> MAHHHHHHSLTAYQASSQARVDAAMHTLFTAPSPELARLYEAMRYSVMNGGKRVRPLLAYAACEALGGKPEQANGAACAVELIHAYSLVHDDLPAMDDDDLRRGQPTTHKAFDEACAILAGDGLQSLAFSALLDPALSDASAEIRLRMVTTLAQAAGPAGMVGGQAIDLGSVGLKLDQQALEYMHRHKTGALIEASVILGALASGRAEKGELKALQTYAQAIGLAFQVQDDILDVESDTATLGKRQGADIARDKPTYPALLGLAAAKEYALELRDQALHALRPFDAAAEPLRE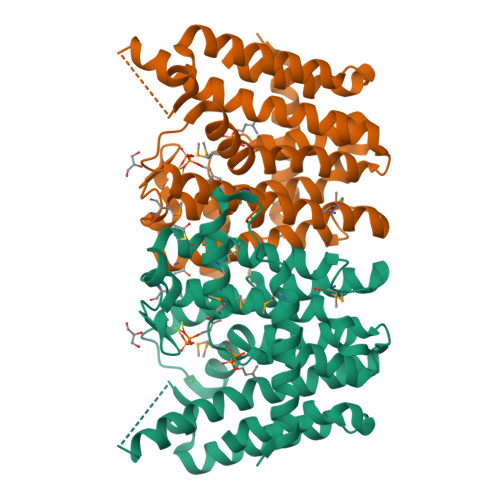LARYIVERRS>[2x]XGCILNGRTDLGTLLFRCRRDSDCPGACICRGNGYCG

Cystine knot peptides (knottins) are small (~4 kDa) peptides characterized by three threaded disulfide bonds arranged in a topological knot; this stabilizing core motif is known as a cystine knot. Solvent exposed loops, that can be bioactive, extend from this knotted core. Here, we describe the development and validation of knottin PET tracers that selectively recognizes human αvβ6 with single-digit nanomolar affinity. Three cystine knot peptides (R01, R01-MG, R01-MR) were engineered for stability, and high-affinity molecular recognition of human αvβ6.

Equilibrium binding assays indicated that all variants bind αvβ6 with low single-digit nanomolar binding affinity (KD~1 nM). As a result of comparative imaging studies in vivo, R01-MG emerged as the lead translational candidate. In addition, the three-dimensional (3D) 1H-NMR solution structure of R01-MG provided evidence that the cystine knot structural element, which defines knottin peptides, was conserved throughout the directed evolution process. Furthermore, x-ray crystallography studies confirmed a disulfide bond pattern consistent with the cystine knot motif. Competition binding assays demonstrated that the N-terminus imaging label, located ~20 Å from the RTDL integrin-recognition motif in active loop-1, did not adversely affect the tracer’s ability to bind αvβ6 with high-affinity. The half-maximal inhibitory concentration (IC50) values for the unlabeled precursor and FP-labeled standard were 0.61 ± 0.31 nM and 0.56 ± 0.46 nM S.D., respectively (Fig. 1c insert). [18F]FP-R01-MG-F2 was evaluated in pre-clinical models with either human αvβ6-positive (~3.5 %ID g−1) or αvβ6-negative (~0.5 %ID g−1) tumors. Selective tracer uptake was demonstrated in the αvβ6 overexpressing tumors. [18F]FP-R01-MG-F2 enables whole lung molecular assessment of lung fibrosis through expression of αvβ6, an ILD histological marker that correlates with prognosis.> EVKQENRLLNESESSSQGLLGYYFSDLNFQAPMVVTSSTTGDLSIPSSELENIPSENQYFQSAIWSGFIKVKKSDEYTFATSADNHVTMWVDDQEVINKASNSNKIRLEKGRLYQIKIQYQRENPTEKGLDFKLYWTDSQNKKEVISSDNLQLPELKQKSSNSRKKRSTSAGPTVPDRDNDGIPDSLEVEGYTVDVKNKRTFLSPWISNIHEKKGLTKYKSSPEKWSTASDPYSDFEKVTGRIDKNVSPEARHPLVAAYPIVHVDMENIILSKNEDQSTQNTDSQTRTISKNTSTSRTHTSEVHGNAEVHASFFDIGGSVSAGFSNSNSSTVAIDHSLSL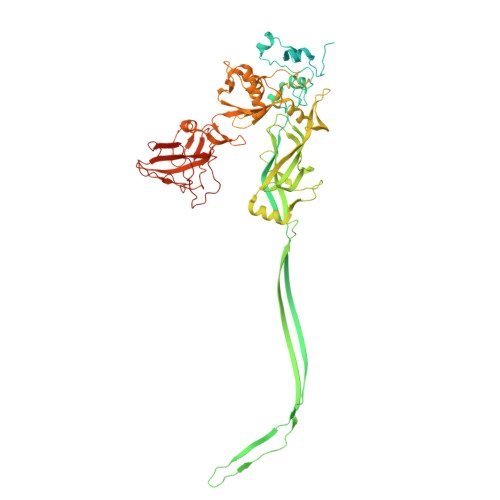AGERTWAETMGLNTADTARLNANIRYVNTGTAPIYNVLPTTSLVLGKNQTLATIKAKENQLSQILAPNNYYPSKNLAPIALNAQDDFSSTPITMNYNQFLELEKTKQLRLDTDQVYGNIATYNFENGRVRVDTGSNWSEVLPQIQETTARIIFNGKDLNLVERRIAAVNPSDPLETTKPDMTLKEALKIAFGFNEPNGNLQYQGKDITEFDFNFDQQTSQNIKNQLAELNATNIYTVLDKIKLNAKMNILIRDKRFHYDRNNIAVGADESVVKEAHREVINSSTEGLLLNIDKDIRKILSGYIVEIEDTEGLKEVINDRYDMLNISSLRQDGKTFIDFKKYNDKLPLYISNPNYKVNVYAVTKENTIINPSENGDTSTNGIKKILIFSKKGYEIG> MRRCSFASTCRYRSADDVPLGLGSAYVWTCRNITSRGQFNPIHNFSYAMERGVRARDVKAFEKLITNPGPLRVAYTPDYLDWLHRCYKAKGTYMDARAVAEKKFNGNIVSSELSAAVNRREGKRGDTRGDTVDNDHHNLPGAPPPGMFLRPAHSFRRLAGELKRRRAQSILDEVARAQGMLDLFERQPHFPAIHIDRCSRFHLVELFKEMVLERSLDSNMIWEKA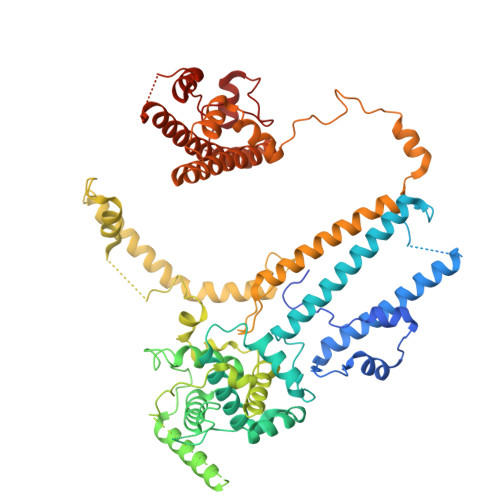LLYRAILSERKPSYPTSFHYIFTAVEDTVFAPTISTPMEMAGSGGEGHDRSSHPLAAKCPTLEAYYYYVYLVKKYYIDNAVEAHVVLRCHREPNAADLLFSNPPPKDDTEIMKAVELLRNADIQRGVAAAAAVSDPTLPPGGEGSVIGNSDNXKNSEKXSEGSRGRPARPPVLPGAYPPIDMLWRCEENLPLLKVLLFGEFNLIVSENPFVKFPSAHGFLTRPYSTDSSRTLADGMSLANVMAEKRGHLLPSLPRNTATSIDARAQDIRRLQQKHHRDDIVSFQKLLRTHAEDSPSAFSSYSDWSYFNPRAVRAEERDRLTRKAVEALKLYDSATNDIYRHSFEDVQACHTQRVTERDRTMPPYLPTLPHFVAIIKKDPHISFLLHIGLPDRNSSEEGSAKHKELEKRIYYLARALYHTALEYHNETVRRVNRQKVNVAASLLDNFVEQEWTTILRDKHDVTDVTKTLNDTQNDKKQLARRLGRYMLFANRSLDDTGFPTDARADDYTRWMAPPSVGKVSL[6-methyl-4-[(~{E})-(oxamoylhydrazinylidene)methyl]-5-oxidanyl-pyridin-3-yl]methyl 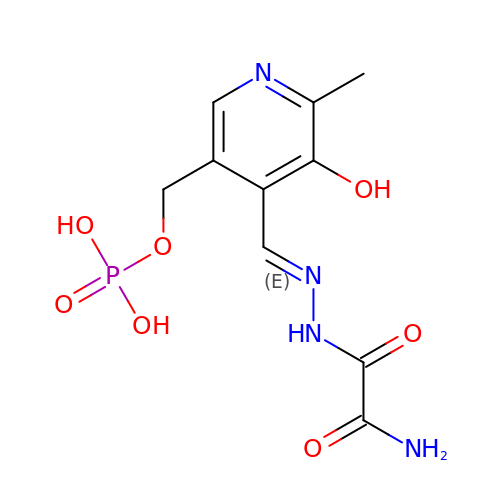dihydrogen phosphate | C10 H13 N4 O7 P | QXOGMDGTZNDNSY-QLKAYGNNSA-N> IVGGRDCAEGECPWQALLVNEENEGFCGGTILNEFYVLTAAHCLHQAKRFTVRVGDRNTEQEEGNEMAH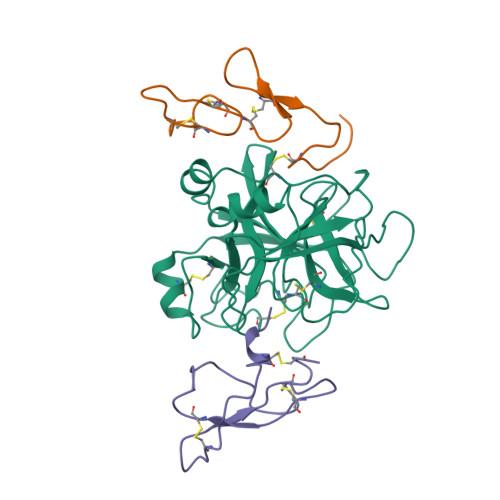EVEMTVKHSRFVKETYDFDIAVLRLKTPIRFRRNVAPACLPEKDWAEATLMTQKTGIVSGFGRTHEKGRLSSTLKMLEVPYVDRSTCKLSSSFTITPNMFCAGYDTQPEDACQGDSGGPHVTRFKDTYFVTGIVSWGEGCARKGKFGVYTKVSNFLKWIDKIMKARAGAAGS;> YNRLCIKPRDWIDECDSNEGGERAYFRNGKGGCDSFWICPEDHTGADYYSSYRDCFNACI;> CSLDNGGCDQFCREERSEVRCSCAHGYVLGDDSKSCVSTERFPCGKFTQGR>MDLAPQMLRELQETNAALQDVRELLRQQVKEITFLKNTV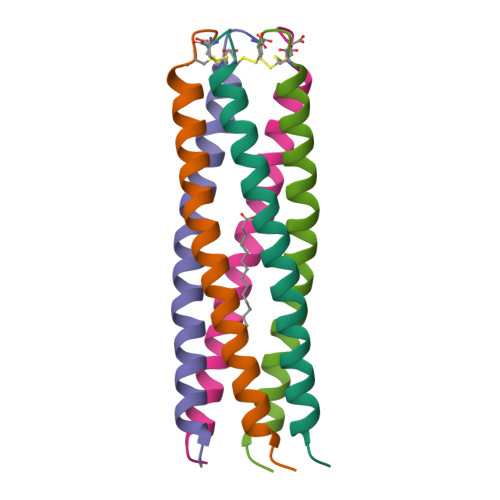MECDAC[5x]(3S,4S,5R)-3-{4-amino-3-fluoro-5-[(2S)-3,3,3-trifluoro-2-hydroxypropyl]benzyl}-5-[(3-tert-butylbenzyl)amino]tetrahydro-2H-thiopyran-4-ol 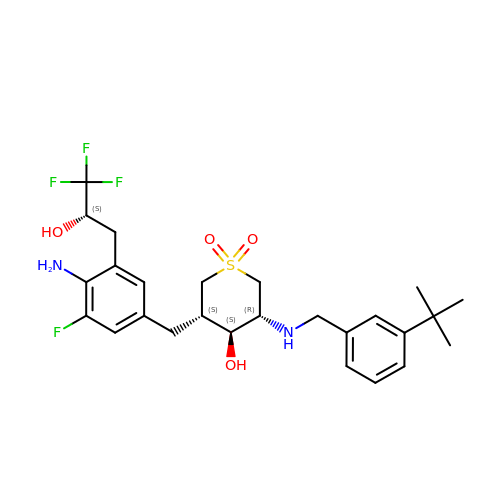1,1-dioxide | C26 H34 F4 N2 O4 S | GCVKLIOGBJALOK-VPJOFFEXSA-N>MTDISQMYDQLSDPFAGLGAGNIHLGYFDGPDDAATLAEAADRLTDQLIARLPVVRDHRVLDVGCGVGKPALRLAGDLGVRVVGVSISEAQIGIANEAARAAGLADRVSFRYADAMRLPFPDASFDGVWAMESLHHMPDRLQALREIARVLRHGGVLSIADFVQLGPVREQDEEALRAFRSGGGVHTLTGIAEYEAEIADAGLTLTSSSDISAN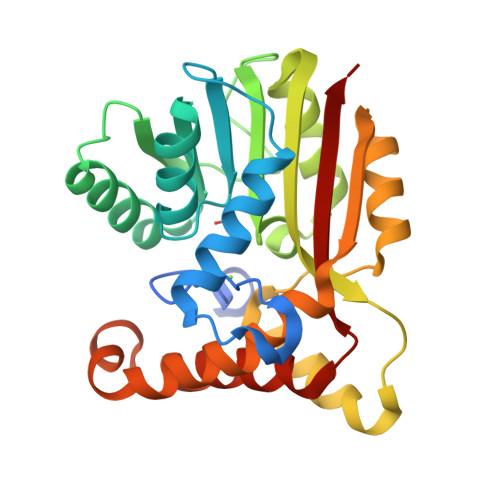VRPSMVRTAEAIRGAADAFLPLMGEEGLRRLIDNFERAATVPQIGYALFAARRS[2x]>GGELMIKSSNAFDVIELSSQIQRYASLSKINNRTNPILKDNKAKEFKDADLKWLKLENCPTAGDVPTTGNNNDLQDQFIACDADYRKGDLSYFGSQFEFSTYVHPSNPEIQRQIKQVVSYFQYRGMERAFIGDAAGYVISEAKKKGFSAQDYRIVLIEPDRVGYFESNAISYEEFIENPSARENFLLKATKDRTLALAVSLAQTGEIAMQRDGSVAFLEDSELCWDTAAGSAKSCLSVRYDTVGNKTELDLKQIDVVSAKGLSFESDGKTKTPVVSTYETFQDGGRAKTINAIECPTGLNNRFAAVVSSFSTAGQNANFSSESAKDSQGTTQKDGSKGPHALLSGISLNWTLTNKVWD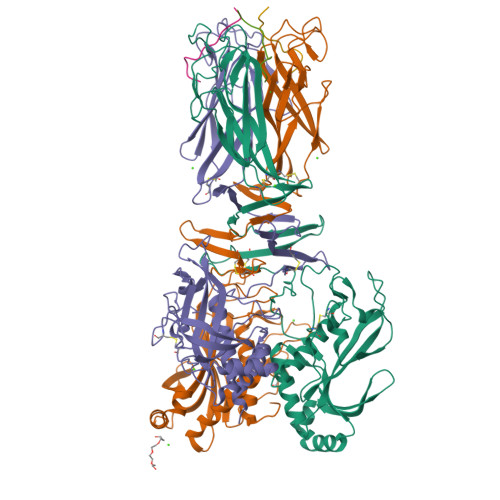VTASIGIESGILPTSGIDSGSLLRNPKSLSFIAFQWCEN[6x];>[6x]FNDNYSSTSTVYATS> 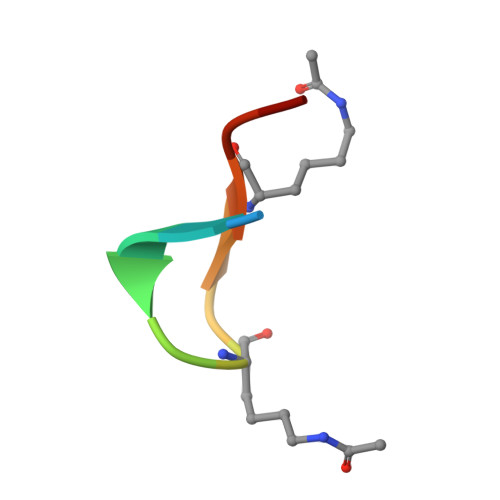XWWIIPKVKKGCX> GAEFKLSDSKTSNIESVPIYSIDEFFLQRKLRSELGYKDTSVIQDLSEKILNDIETLEHNPVALEQKLVDLLKFENISLAEFILKNRSTIFWGIRLAKSTENEIPN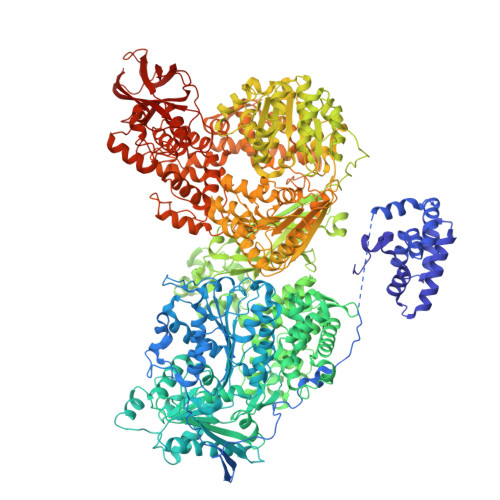LIEKMVAKGLNDLVEQYKFRETTHSKRELDSGDDQPQSSEAKRTKFSNPAIPPVIDLEKIKFDESSKLMTVTKVSLPEGSFKRVKPQYDEIHIPAPSKPVIDYELKEITSLPDWCQEAFPSSETTSLNPIQSKVFHAAFEGDSNMLICAPTGSGKTNIALLTVLKALSHHYNPKTKKLNLSAFKIVYIAPLKALVQEQVREFQRRLAFLGIKVAELTGDSRLSRKQIDETQVLVSTPEKWDITTRNSNNLAIVELVRLLIIDEIHLLHDDRGPVLESIVARTFWASKYGQEYPRIIGLSATLPNYEDVGRFLRVPKEGLFYFDSSFRPCPLSQQFCGIKERNSLKKLKAMNDACYEKVLESINEGNQIIVFVHSRKETSRTATWLKNKFAEENITHKLTKNDAGSKQILKTEAANVLDPSLRKLIESGIGTHHAGLTRSDRSLSEDLFADGLLQVLVCTATLAWGVNLPAHTVIIKGTDVYSPEKGSWEQLSPQDVLQMLGRAGRPRYDTFGEGIIITDQSNVQYYLSVLNQQLPIESQFVSKLVDNLNAEVVAGNIKCRNDAVNWLAYTYLYVRMLASPMLYKVPDISSDGQLKKFRESLVHSALCILKEQELVLYDAENDVIEATDLGNIASSFYINHASMDVYNRELDEHTTQIDLFRIFSMSEEFKYVSVRYEEKRELKQLLEKAPIPIREDIDDPLAKVNVLLQSYFSQLKFEGFALNSDIVFIHQNAGRLLRAMFEICLKRGWGHPTRMLLNLCKSATTKMWPTNCPLRQFKTCPVEVIKRLEASTVPWGDYLQLETPAEVGRAIRSEKYGKQVYDLLKRFPKMSVTCNAQPITRSVMRFNIEIIADWIWDMNVHGSLEPFLLMLEDTDGDSILYYDVLFITPDIVGHEFTLSFTYELKQHNQNNLPPNFFLTLISENWWHSEFEIPVSFNGFKLPKKFPPPTPLLENISISTSELGNDDFSEVFEFKTFNKIQSQVFESLYNSNDSVFVGSGKGTGKTAMAELALLNHWRQNKGRAVYINPSGEKIDFLLSDWNKRFSHLAGGKIINKLGNDPSLNLKLLAKSHVLLATPVQFELLSRRWRQRKNIQSLELMIYDDAHEISQGVYGAVYETLISRMIFIATQLEKKIRFVCLSNCLANARDFGEWAGMTKSNIYNFSPSERIEPLEINIQSFKDVEHISFNFSMLQMAFEASAAAAGNRNSSSVFLPSRKDCMEVASAFMKFSKAIEWDMLNVEEEQIVPYIEKLTDGHLRAPLKHGVGILYKGMASNDERIVKRLYEYGAVSVLLISKDCSAFACKTDEVIILGTNLYDGAEHKYMPYTINELLEMVGLASGNDSMAGKVLILTSHNMKAYYKKFLIEPLPTESYLQYIIHDTLNNEIANSIIQSKQDCVDWFTYSYFYRRIHVNPSYYGVRDTSPHGISVFLSNLVETCLNDLVESSFIEIDDTEAEVTAEVNGGDDEATEIISTLSNGLIASHYGVSFFTIQSFVSSLSNTSTLKNMLYVLSTAVEFESVPLRKGDRALLVKLSKRLPLRFPEHTSSGSVSFKVFLLLQAYFSRLELPVDFQNDLKDILEKVVPLINVVVDILSANGYLNATTAMDLAQMLIQGVWDVDNPLRQIPHFNNKILEKCKEINVETVYDIMALEDEERDEILTLTDSQLAQVAAFVNNYPNVELTYSLNNSDSLISGVKQKITIQLTRDVEPENLQVTSEKYPFDKLESWWLVLGEVSKKELYAIKKVTLNKETQQYELEFDTPTSGKHNLTIWCVCDSYLDADKELSFEINVK>[2x]DGTSQ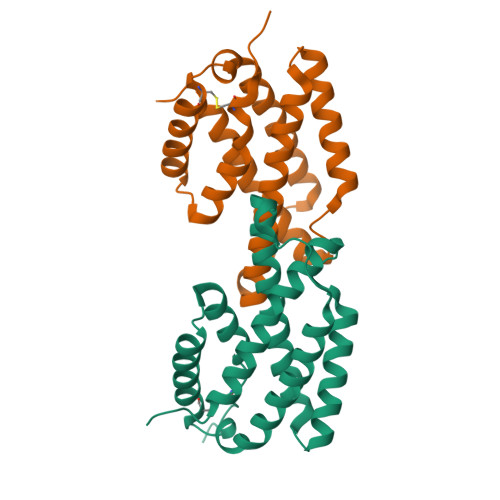LAELVDAAAERLEVADPVAAFKWRAQLPIEDSGRVEQQLAKLGEDARSQHIDPDYVTRVFDDQIRATEAIEYSRFSDWKLNPASAPPEPPDLSASRSAIDSLNNRMLSQIWSHWSLLSAPSCAAQLDRAKRDIVRSRHLDSLYQRALTTATQSYCQALPPA>MQGSVTEFLKPRLVDIEQVSSTHAKVTLEPLERGFGHTLGNALRRILLSSMPGCAVTEVEIDGVLHEYSTKEGVQEDILEILLNLKGLAVRVQGKDEVILTLNKSGIGPVTAADITHDGDVEIVKPQHVICHLTDENASISMRIKVQRGRGYVPASTRIHSEEDERPIGRLLVDACYSPVERIAYNVEAARVEQRTDLDKLVIEMETNGTIDPEEAIRRAATILAEQLEAFVDLRDVRQPEVKEEKPEFDPILLRPVDDLELTVRSANCLKAEAIHYIGDLVQRTEVELLKTPNLGKKSLTEIKDVLASRGLSLGMRLENWPPASIADE[2x];> MVYSYTEKKRIRKDFGKRPQVLDVPYLLSIQLDSFQKFIEQDPEGQYGLEAAFRSVFPIQSYSGNSELQYVSYRLGEPVFDVQECQIRGVTYSAPLRVKLRLVIYEREAPEGTVKDIKEQEVYMGEIPLMTDNGTFVINGTERVIVSQLHRSPGVFFDSDKGKTHSSGKVLYNARIIPYRGSWLDFEFDPKDNLFVRIDRRRKLPATIILRALNYTTEQILDLFFEKVIFEIRDNKLQMELVPERLRGETASFDIEANGKVYVEKGRRITARHIRQLEKDDVKLIEVPVEYIAGKVVAKDYIDESTGELICAANMELSLDLLAKLSQSGHKRIETLFTNDLDHGPYISETLRVDPTNDRLSALVEIYRMMRPGEPPTREAAESLFENLFFSEDRYDLSAVGRMKFNRSLLREEIEGSGILSKDDIIDVMKKLIDIRNGKGEVDDIDHLGNRRIRSVGEMAENQFRVGLVRVERAVKERLSLGDLDTLMPQDMINAKPISAAVKEFFGSSQLSQFMDQNNPLSEITHKRRISALGPGGLTRERAGFEVRDVHPTHYGRVCPIETPEGPNIGLINSLSVYAQTNEYGFLETPYRKVTDGVVTDEIHYLSAIEEGNYVIAQANSNLDEEGHFVEDLVTCRSKGESSLFSRDQVDYMDVSTQQVVSVGASLIPFLEHDDANRALMGANMQRQAVPTLRADKPLVGTGMERAVAVDSGVTAVAKRGGVVQYVDASRIVIKVNEDEMYPGEAGIDIYNLTKYTRSNQNTCINQMPCVSLGEPVERGDVLADGPSTDLGELALGQNMRVAFMPWNGYNFEDSILVSERVVQEDRFTTIHIQELACVSRDTKLGPEEITADIPNVGEAALSKLDESGIVYIGAEVTGGDILVGKVTPKGETQLTPEEKLLRAIFGEKASDVKDSSLRVPNGVSGTVIDVQVFTRDGVEKDKRALEIEEMQLKQAKKDLSEELQILEAGLFSRIRAVLVAGGVEAEKLDKLPRDRWLELGLTDEEKQNQLEQLAEQYDELKHEFEKKLEAKRRKITQGDDLAPGVLKIVKVYLAVKRRIQPGDKMAGRHGNKGVISKINPIEDMPYDENGTPVDIVLNPLGVPSRMNIGQILETHLGMAAKGIGDKINAMLKQQQEVAKLREFIQRAYDLGADVRQKVDLSTFSDEEVMRLAENLRKGMPIATPVFDGAKEAEIKELLKLGDLPTSGQIRLYDGRTGEQFERPVTVGYMYMLKLNHLVDDKMHARSTGSYSLVTQQPLGGKAQFGGQRFGEMEVWALEAYGAAYTLQEMLTVKSDDVNGRTKMYKNIVDGNHQMEPGMPESFNVLLKEIRSLGINIELEDE;> VKDLLKFLKAQTKTEEFDAIKIALASPDMIRSWSFGEVKKPETINYRTFKPERDGLFCARIFGPVKDYECLCGKYKRLKHRGVICEKCGVEVTQTKVRRERMGHIELASPTAHIWFLKSLPSRIGLLLDMPLRDIERVLYFESYVVIEGGMTNLERQQILTEEQYLDALEEFGDEFDAKMGAEAIQALLKSMDLEQECEQLREELNETNSETKRKKLTKRIKLLEAFVQSGNKPEWMILTVLPVLPPDLRPLVPLDGGRFATSDLNDLYRRVINRNNRLKRLLDLAAPDIIVRNEKRMLQEAVDALLDNGRRGRAITGSNKRPLKSLADMIKGKQGRFRQNLLGKRVDYSGRSVITVGPYLRLHQCGLPKKMALELFKPFIYGKLELRGLATTIKAAKKMVEREEAVVWDILDEVIREHPVLLNRAPTLHRLGIQAFEPVLIEGKAIQLHPLVCAAYNADFDGDQMAVHVPLTLEAQLEARALMMSTNNILSPANGEPIIVPSQDVVLGLYYMTRDCVNAKGEGMVLTGPKEAERLYRSGLASLHARVKVRITEYEKDANGELVAKTSLKDTTVGRAILWMIVPKGLPYSIVNQALGKKAISKMLNTCYRILGLKPTVIFADQIMYTGFAYAARSGASVGIDDMVIPEKKHEIISEAEAEVAEIQEQFQSGLVTAGERYNKVIDIWAAANDRVSKAMMDNLQTETVINRDGQEEKQVSFNSIYMMADSGARGSAAQIRQLAGMRGLMAKPDGSIIETPITANFREGLNVLQYFISTHGARKGLADTALKTANSGYLTRRLVDVAQDLVVTEDDCGTHEGIMMTPVIEGGDVKEPLRDRVLGRVTAEDVLKPGTADILVPRNTLLHEQWCDLLEENSVDAVKVRSVVSCDTDFGVCAHCYGRDLARGHIINKGEAIGVIAAQSIGEPGTQLTMRTFHIGGAASRAAAESSIQVKNKGSIKLSNVKSVVNSSGKLVITSRNTELKLIDEFGRTKESYKVPYGAVLAKGDGEQVAGGETVANWDPHTMPVITEVSGFVRFTDMIDGQTITRQTDELTGLSSLVVLDSAERTAGGKDLRPALKIVDAQGNDVLIPGTDMPAQYFLPGKAIVQLEDGVQISSGDTLARIPQESGGTKDITGGLPRVADLFEARRPKEPAILAEISGIVSFGKETKGKRRLVITPVDGSDPYEEMIPKWRQLNVFEGERVERGDVISDGPEAPHDILRLRGVHAVTRYIVNEVQDVYRLQGVKINDKHIEVIVRQMLRKATIVNAGSSDFLEGEQVEYSRVKIANRELEANGKVGATYSRDLLGITKASLATESFISAASFQETTRVLTEAAVAGKRDELRGLKENVIVGRLIPAGTGYAYHQDRMRRRAAGEAPAAPQVTAEDASASLAELLNAGLGGSDNELEVHHHHHH;> MARVTVQDAVEKIGNRFDLVLVAARRARQMQVGGKDPLVPEENDKTTVIALREIEEGLINNQILDVRERQEQQEQEAAELQAVTAIAEGRR;> GHMQSWYLLYCKRGQLQRAQEHLERQAVNCLAPMITLEKIVRGKRTAVSEPLFPNYLFVEFDPEVIHTTTINATRGVSHFVRFGASPAIVPSAVIHQLSVYKPKDIVDPATPYPGDKVIITEGAFEGFQAIFTEPDGEARSMLLLNLINKEIKHSVKNTEFRKL

RfaH, a paralog of the universally conserved NusG, binds to RNA polymerases (RNAP) and ribosomes to activate expression of virulence genes. In free, autoinhibited RfaH, an α-helical KOW domain sequesters the RNAP-binding site. Upon recruitment to RNAP paused at an ops site, KOW is released and refolds into a β-barrel, which binds the ribosome. RfaH recruitment requires a 12-nucleotide (nt) operon polarity suppressor (ops) sequence, which induces RNAP pausing.

To answer this question, we subjected opsPECRec after NTP addition and heating (37 oC) to cryoEM/SPA, yielding a cryoEM reconstruction at 3.0 Å resolution. The resulting complex was nearly identical to opsPECRec with a major exception: a clear additional density in the secondary channel showed that the transcript had been elongated by at least two nts followed by RNAP backtracking. These findings establish that opsPECRec is elongation-competent (i.e., can transiently adopt a post-translocated state) and that, following nucleotide addition, RNAP slides back, generating opsPECBack. Third, we present a structure of RfaH fully engaged with RNAP in an even deeper paused state, which is likely necessary to recruit the pioneering ribosome. Fourth, we present a structure that captures an unsuccessful attempt of RfaH-bound RNAP to escape the recruitment site, leading to a backtracked state which is rescued by accessory factors. We do not observe scrunching, but the transition to opsPECBack must be accompanied by at least two translocation steps and likely requires scrunching, as proposed earlier.> MSNQGEYPEDNRVGKHEPHDLSLTRRDLIKVSAATAATAVVYPHSTLAASVPAATPAPEIMPLTLKVNGKTEQLEVDTRTTLLDTLRENLHLIGTKKGCDHGQCGACTVLVNGRRLNACLTLAVMHQGAEITTIEGLGSPDNLHPMQAAFIKHDGFQCGYCTSGQICSSVAVLKEIQDGIPSHVTVDLVSAPETTADEIRERMSGNICRCGAYANILAAIEDAAGEIKS;> MKAFTYERVNTPAEAALSAQRVPGAKFIAGGTNLLDLMKLEIETPTHLIDVNGLGLDKIEVTDAGGLRIGALVRNTDLAAHERVRRDYAVLSRALLAGASGQLRNQATTAGNLLQRTRCPYFYDTNQPCNKRLPGSGCAALEGFSRQHAVVGVSEACIATHPSDMAVAMRLLDAVVETITPEGKTRSITLADFYHPPGKTPHIETALLPGELIVAVTLPPPLGGKHIYRKVRDRASYAFALVSVAAIIQPDGSGRVALGGVAHKPWRIEAADAQLSQGAQAVYDTLFASAHPTAENTFKLLLAKRTLASVLAEARAQA;> MKFDKPAGENPIDQLKVVGRPHDRIDGPLKTTGTARYAYEWHEEAPNAAYGYIVGSAIAKGRLTALDTDAAQKAPGVLAVITASNAGVLGKGDKNTARLLGGPTIEHYHQAIALVVAETFEQARAAASLVQAHYRRNKGAYSLADEKQAVNQPPEDTPDKNVGDFDGAFTSAAVKIDATYTTPDQSHMAMEPHASMAVWD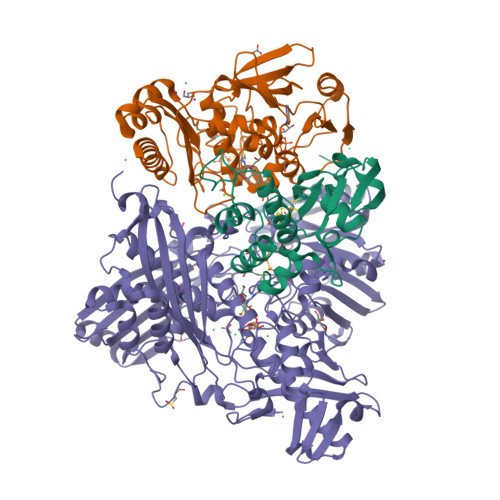GNKLTLWTSNQMIDWCRTDLAKTLKVPVENVRIISPYIGGGFGGKLFLRSDALLAALAARAVKRPVKVMLPRPSIPNNTTHRPATLQHLRIGADQSGKITAISHESWSGNLPGGTPETAVQQSELLYAGANRHTGLRLATLDLPEGNAMRAPGEAPGLMALEIAIDELAEKAGIDPVEFRILNDTQVDPAGPTRCFSRRQLIECLRTGADKFGWKQRNATPGQVRDGEWLVGHGVAAGFRNNLLEKSGARVHLEQNGTVTVETDMTDIGTGSYTILAQTAAEMLGVPLEQVAVHLGDSSFPVSAGSGGQWGANTSTSGVYAACMKLREMIASAVGFDPEQSQFADGKITNGTRSATLHEATAGGRLTAEESIEFGTLSKEYQQSTFAGHFVEVGVHSATGEVRVRRMLAVCAAGRILNPKTARSQVIGAMTMGMGAALMEELAVDDRLGYFVNHDMAGYEVPVHADIPKQEVIFLDDTDPISSPMKAKGVGELGLCGVSAAIANAVYNATGIRVRDYPITLDKLLDKLPDVV>SSQKSQFAYRSSKSIGLVNASENYASPPKFEAISEPARNACYSPNGKLFAYATATQVVINDTESGAKLTQLPAANTYELGFSPLGKYLSTWERPGKEADGTPKQNMKVWNTETGQLVFSFVQRNQTGWNLQYTCDESLAARLVTNEVHFYETGNMSKGPIAKLRVEGISDFALSPGQNHAVAVFIPEKKGAPASVRTYSIPNFNSPLSQKTFFKADKVQFKWNALGTSLLVLTQTEVDKSNKNYYGETNLYLLGITGQFDCRVDLDREGPIHDVCWNADSKEFGIVYGYMPAKTAIFDNRANVVSIIPPAPRNTLIFSPNSRYILLAGFGNLQGSIDIFDAANNMKKITTVEAANCTYCEFSPDSQFLLTAVTSPRLRVDNSIKIWHITGAPMFYEEFNELYQAFWRPRPLN[2x]

The eukaryotic translation initiation factor 2A (eIF2A) was identified as a factor that stimulates the binding of methionylated initiator tRNA (Met-tRNAiMet) to the 40S ribosomal subunit, but its physiological role remains poorly defined. Recently, eIF2A was shown to be involved in unconventional translation initiation from CUG codons and in viral protein synthesis under stress conditions where eIF2 is inactivated. Based on these findings, eIF2A might be a tRNA-loading factor in unconventional translation initiation events, such as non-AUG translation initiation, and an alternative factor of eIF2 when the active eIF2 is limited, due to the stress response by eIF2 kinases. eIF2A is predicted to contain two to four WD-repeats at the N-terminus and a coiled-coil at the C-terminus, but this prediction has not been structurally confirmed.

Since the C-terminal region of eIF2A is predicted to be highly disordered, we prepared a C-terminally truncated eIF2A (residues 1–424). We determined the crystal structure of the C-terminally truncated eIF2A at 2.5 Å resolution. The final model consists of residues 3–234, 242–248, and 256–412. The crystal structure of the truncated eIF2A revealed that it adopts a nine-bladed β-propeller fold, with the same overall topology as the regular β-propeller proteins, involving circularly arranged repeats of a four-stranded antiparallel β-sheet motif. There are two molecules of eIF2A-WD in the asymmetric unit, and no significant structural differences exist between them (the root-mean-square deviation is 0.98 Å for 391 Cα atoms), except for blade 6. The electron density of blade 6 is not well-defined, as compared to the other blades, due to either the crystal packing or the flexible nature of this blade (data not shown). However, the central channel of eIF2A-WD has an inverted structure, with the wider opening at the top and the narrower opening at the bottom. Furthermore, the opening at the bottom face is constricted by the inward twists of the AB loops in eIF2A-WD. A phylogenetic analysis revealed that the surface residues on the top face of eIF2A-WD, including these loops, are highly conserved, in contrast to the abundance of non-conserved residues on the bottom face. Especially, the residues at the top faces of blades 6–9 showed strong conservation. This highly conserved top face is positively charged, and the most positively-charged regions are the grooves between blades 3–4 and between blades 6–7.>MVMALKPIKLYTAPTPNGYKISIFLEVLGLDYEVQKFDLSKNETKEDWFVKLNPNGRIPTINDPNFKGVDGGLVLSQTGAILQYLADTYDKEHKFSYPAGTAEYYKTLEYLIFQVAENGPIQGQANHFVFAAKEKVPYGINRYITDTKRIYGVFE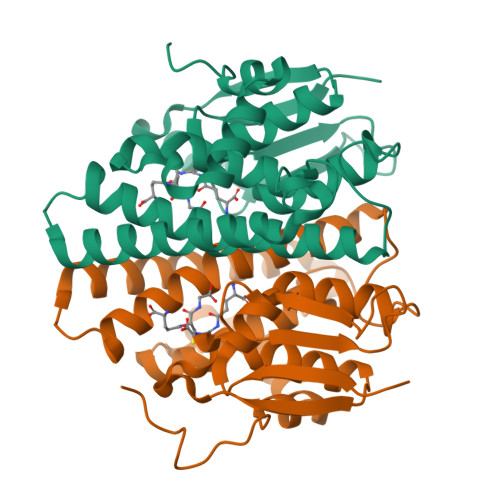DILSRNKANDSKYLVGDRYTVADFALLGWAYRLSRLEIDINQWPLLGKWYDSLLKLPAVQKGFEVPPKNAENLYFQ[8x]> MAHHHHHHAVTSDESVSAGNYYNANYLESYASKAYNESGLGSVYSKTSTTWKTWSPDASSVKLKLYTTGSDNEAGASAIGTYDMKKDSSTGVWSLNLSGDYKNKYYTYLVTVNGTTKETQDVYSQAVGVNGNRTMVVDLDSTDPSGWSDDKHVLFNSASEAAVWEVHVRDFSVSKNSGVSEDNKGKYLAFAEGGTTLNSDTSSSAVSTGIDYLVEQGINCVQLMPVYDYGSVKEDVASSSSNRNWGYDPVNYNAPEGSYSTNPYDGNTRITEFKQMIQALHDRGISVVMDVVYNHTFSNDSCFNRTVPGYYYRMHSSSAYSNGSGCGNETASDKLMYRKYMIESVKYWAEEYHIDGFRFDLMGIHDITTMNDIRSALDGLYSDGSGKKILMYGEPWTGGSVAISDGCSQSKAGSLNPRVGMFCDSYRDAIKGSTDGSDKGFVQGNTDKAGTVANGVTGKGFSAQAPSQTIAYADAHDNLILWDKIVKSNGSSSWNSTSSSLRGQVKKVMGLLLTSQGIPFMTAGSEFCRTKQGDTNSYKSSDAINEIDWSRVKTYSDVAAYYKGLLEIRENYSPMKSSTFNTPSFQSTHGDVVAYTYSNNKSNEWGKVCVLVNASSTNDWPITLDGSGWTVVADGTTAGLKSLGTVSGNTYTVPANSACVLVQSSTFNNLKVSEKTFGTVTIKHIDDSGNVLKTSTAKYADGTTYRTYPDTTILYDYALKDTQGVTSGTVTGGKNYNVTYVYSSSGIRSGYVTVNYVDENGESIKDTVSTKYREGDSYSVPFTSIQGYQLDTDKYPANTTGTFNGTNTTINFVYKALDSTSSVVHYYNSNNWSNVRCYAYTDGGEEPNGKWNNATVMTSEGNGWL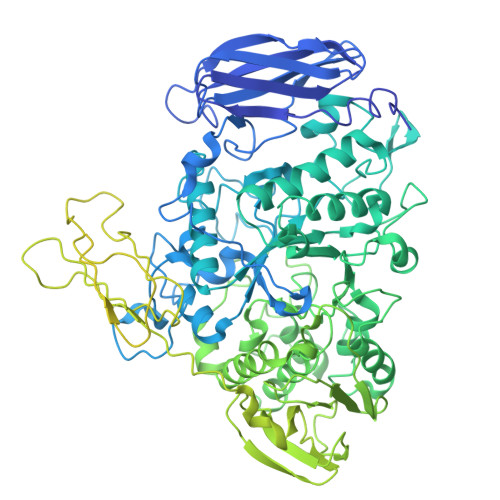KCTIPASSSYVMFHTDSQQEPGANETGYLVSGEAWIQNKKLSFSSKVITSHIDAATGEKIADDEILIQSKVSSDDTYKTSPLSGRTDVIAPVNASGNLSSGIINVVYLYTSSERPSTAPSTVTPTTAPVTQPTEKILIGDVNLNGAIDIVDTTAVQKYIVKLITLSDKALIAAARCDADGENDIVSVKDATYIQMYVAKLDGHGNVGTYYESEVTPTTAPVTEPATEEPTVAPTTVPVTTAPVTEPTTTPSSTYTVKFTDSLNWDGTLYCYSWAEDGTSTKSWPGVAMTYLNTNDYGQKVYSVEVPNTVDYIIFTNGSSQTIDIGFDGTSLNYYTESQYDSKGHAYVGSW> GSLVPELNEKDDDQVQKALASRENTQLMNRDNIEITVRDFKTLAP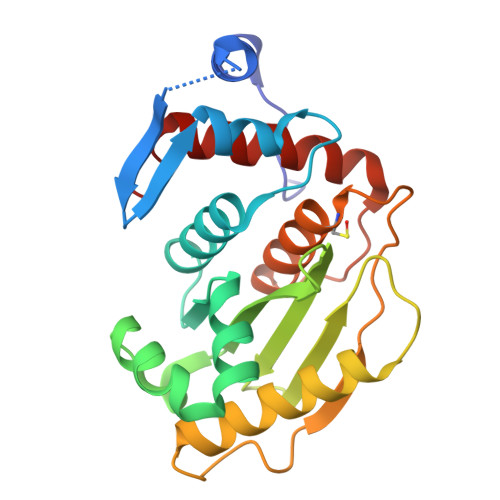RRWLNDTIIEFFMKYIEKSTPNTVAFNSFFYTNLSERGYQGVRRWMKRKKTQIDKLDKIFTPINLNQSHWALGIIDLKKKTIGYVDSLSNGPNAMSFAILTDLQKYVMEESKHTIGEDFDLIHLDCPQQPNGYDCGIYVCMNTLYGSADAPLDFDYKDAIRMRRFIAHLILTDALK> MAEEEEVEEGRSSSSAILDLPEPLLLHILSFLTDVRSRHRAALACGRMRAAERATRSELSLRGDPRSPGFLFLSHAFRFPALEHLDLSLVSPWGHPLLSSVPPCGGGGGGAPSASSSSGMNVYHPEAISEQNAFIAARLAGCFPAVTSLAVYCRDPTTLANLTPHWQASLRRVKLVRWHQRPPTLPDGADLEPLLETCAALRELDLSEFYCWTEDVVRALTTHPSATAALTHLDLGLAAATDGFKSSELGPIAASCPNLRKLVAPCLFNPRFSDCVGDDALLSLATSCPRLTVLRLSEPFEAAANIQREEAAITVAGLVAFFAALPALEDFTMDLQHNVLEAAPAMEALARRCPRIKFLTLGSFQGLCKASWLHLDGVAVCGGLESLYMKNCQDLTDASLAAIGRGCRRLAKFGIHGCDLVTSAGIRRLAF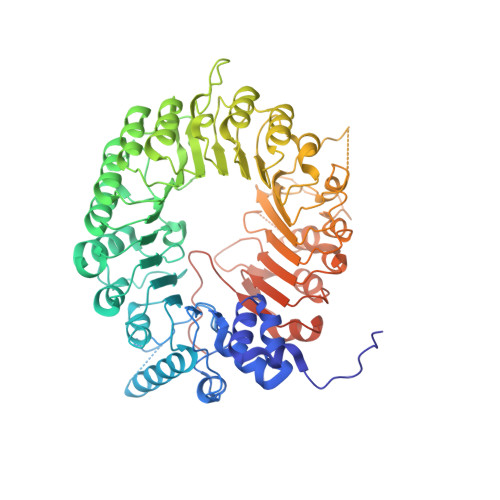TLRPTLKEVTVLHCRLLHTAECLTALSPIRDRIESLEINCVWNTTENLYFQSLGSWEMLRSLSLWFSAGQLLSPLISAGLDSCPVLEEISIKVEGDCRTCPRPAPRTIFGLSDLAGFPVLAKMKLDLSEAVGYALTAPTGQMDLSLWERFYLHGIESLQTLYELDYWPPQDKDVHHRSLTLPAVGLIQRCVGLRKLFIHGTTHEHFMTFFLSIPNLRDMQLREDYYPAPENDLMFTEMRAESWLRFEVQLNSRQIDD>[2x]MADLNQRRQRSEFQSKIKILLSTTIKAKPELVPSLLKLALNDAMTYDKATKSGGANGSIRFSSELS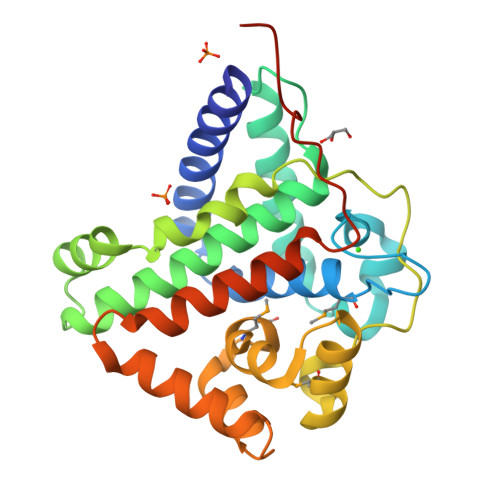RAENEGLSDGLSLIEEVKKEIDSISKGGPISYADIIQLAGQSAVKFTYLASAIRKCGGNEEKGNLLYTAYGSAGQWGLFDRNFGRSDATEADPEGRVPQWGKATVQEMKDKFIAVGLGPRQLAVMSAFLGPDQAATEQLLATDPQVAPWVQKYQRSRETVSQTDYEVDLITAFTKLSCLGQQINFEAYTYPVERINLSKLKL> AHHHHHHSAALEVLFQGPGMMAKNNKTTEAKMSKKRAASEESDVEEDEDKLLSVDGLIDAEASESDEDDDEYESAVEEKESSSDKEAQDDSDDDSDAELNKLLAEEEGDGEEDYDSSEFSDDTTSLTDRLSGVKLQTIVDPNIYSKYADGSDRIIKPEINPVYDSDDSDAETQNTIGNIPLSAYDEMPHIGYDINGKRIMRPAKGSALDQLLDSIELPEGWTGLLDKNSGSSLNLTKEELELISKIQRNEQTDDSINPYEPLIDWFTRHEEVMPLTAVPEPKRRFVPSKNEAKRVMKIVRAIREGRIIPPKKLKEMKEKEKIENYQYDLWGDSTETNDHVMHLRAPKLPPPTNEESYNPPEEYLLSPEEKEAWENTEYSERERNFIPQKYSALRKVPGYGESIRERFERSLDLYLAPRVRKNKLNIDPNSLIPELPSPKDLRPFPIRCSTIYAGHKGKVRTLSIDPSGLWLATG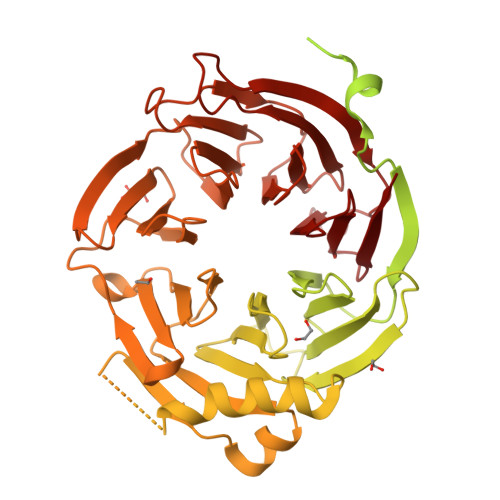SDDGTVRVWEILTGREVYRTTLIDDEENPDYHIECIEWNPDANNGILAVAVGENIHLIVPPIFGYDIENNGKTKIEDGFGYDTFGTVKKSNLEVNENGDGDEDGENESAKNAVKKQVAQWNKPSQKQLEKDICITISCKKTVKKLSWHRKGDYFVTVQPDSGNTSVLIHQVSKHLTQSPFKKSKGIIMDAKFHPFKPQLFVCSQRYVRIYDLSQQILVKKLLPGARWLSKIDIHPRGDNLIASSFDKRVLWHDLDLASTPYKTLRYHEKAVRSVNFHKKLPLFSSAADDGTIHVFHATVYDDMMKNPMIVPLKKLTGHKVINSLGVLDAIWHPREAWLFSAGADNTARLWTT> SNADDYTAGKEYVELSSPVPVSQPGKIEVVELFWYGCPHCYAFEPTIVPWSEKLPADVHFVRLPALFGGIWNVHGQMFLTLISMGVEHDVHNAVFEAIHKEHKKLATPEEMADFLAGKGVDKEKFLSTYNSFAIKGQMEKAKKLAMAYQVTGVPTMVVNGKYRFDIGSAGGPEETLKLADYLIEK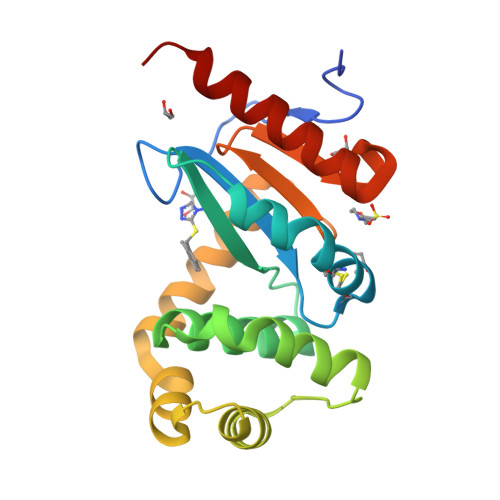ERAAAKK2-deoxy-2-({[(1,1-dioxido-1-benzothiophen-2-yl)methoxy]carbonyl}amino)-beta-D-glucopyranose 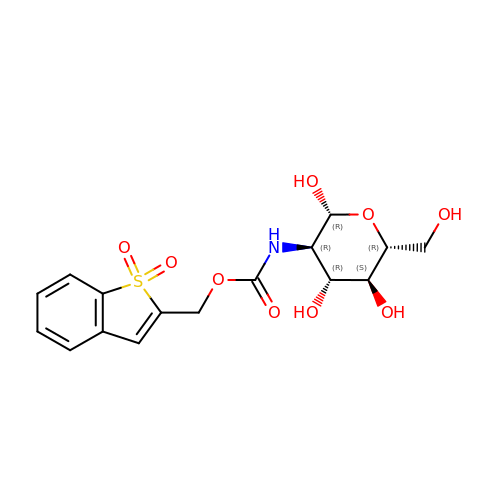| C16 H19 N O9 S | ACIPDYFLRJNHEW-DIAXPKBXSA-N> MELQQNFTDNNSIKYTCILILIAFAFSVLCRLYWVAWASEFYEFFFNDQLMITTNDGYAFAEGARDMIAGFHQPNDLSYFGSSLSTLTYWLYSILPFSFESIILYMSTFFASLIVVPIILIAREYKLTTYGFIAALLGSIANSYYNRTMSGYYDTDMLVLVLPMLILLTFIRLTINKDIFTLLLSPIFIMIYLWWYPSSYSLNFAMIGLFGLYTLVFHRKEKIFYLAIALMIIALSMLAWQYKLALIVLLFAIFAFKEEKINFYMIWALIFISISILHLSGGLDPVLYQLKFYVFKASDVQNLKDAAFMYFNVNETIMEVNTIDPEVFMQRISSSVLVFILSFIGFILLCKDHKSMLLALPMLALGFMALRAGLRFTIYAVPVMALGFGYFLYAFFNFLEKKQIKLSLRNKNILLILIAFFSISPALMHIYYYKSSTVFTSYEASILNDLKNKAQREDYVVAWWDYGYPIRYYSDVKTLIDGGKHLGKDNFFSSFVLSKEQ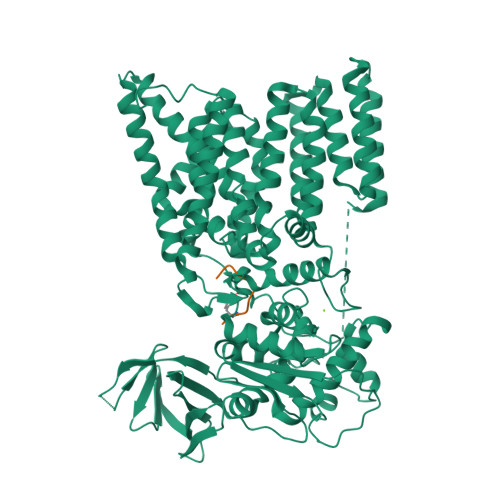IPAANMARLSVEYTEKSFKENYPDVLKAMVKDYNQTSAKDFLESLNDKNFKFDTNKTRDVYIYMPYRMLRIMPVVAQFANTNPDNGEQEKSLFFSQANAIAQDKTTGSVMLDNGVEIINDFRALKVEGASIPLKAFVDIESITNGKFYYNEIDSKAQIYLLFLREYKSFVILDESLYNSAYIQMFLLNQYDQDLFEQVTNDTRAKIYRLKREFHHHHHHHHHH;> GDQNATFG>[2x]RSPWEENFSRSYPCDEKKQNDSVIAECSNRRLQEVPQTVGKYVTELDLSDNFITHITNESFQGLQNLTKINLNHNPNVQHQNGNPGIQSNGLNITDGAFLNLKNLRELLLEDNQLPQIPSGLPESLTELSLIQNNIYNITKEGISRLINLKNLYLAWNCYFNKVCEKTNIEDGVFETLTNLELLSLSFNSLSHVPPKLPSSLRKLFLSNTQIKYISEEDFK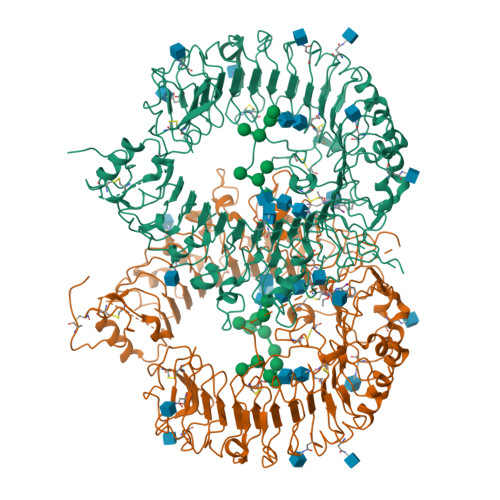GLINLTLLDLSGNCPRCFNAPFPCVPCDGGASINIDRFAFQNLTQLRYLNLSSTSLRKINAAWFKNMPHLKVLDLEFNYLVGEIASGAFLTMLPRLEILDLSFNYIKGSYPQHINISRNFSKLLSLRALHLRGYVFQELREDDFQPLMQLPNLSTINLGINFIKQIDFKLFQNFSNLEIIYLSENRISPLVKDTRQSYANSSSFQRHIRKRRSTDFEFDPHSNFYHFTRPLIKPQCAAYGKALDLSLNSIFFIGPNQFENLPDIACLNLSANSNAQVLSGTEFSAIPHVKYLDLTNNRLDFDNASALTELSDLEVLDLSYNSHYFRIAGVTHHLEFIQNFTNLKVLNLSHNNIYTLTDKYNLESKSLVELVFSGNRLDILWNDDDNRYISIFKGLKNLTRLDLSLNRLKHIPNEAFLNLPASLTELHINDNMLKFFNWTLLQQFPRLELLDLRGNKLLFLTDSLSDFTSSLRTLLLSHNRISHLPSGFLSEVSSLKHLDLSSNLLKTINKSALETKTTTKLSMLELHGNPFECTCDIGDFRRWMDEHLNVKIPRLVDVICASPGDQRGKSIVSLELTTCVSDVTEFLVPR>ASQHHHHHHVTNDCPVTITTTPPQTVGVSSTTPIGFSAKVTTSDQCIKAGAKVWLWGTGPANKWVLQHAKVAKQKYTLNPSIDGGADFVNQGTDAKIYKKLTSGNKFLNASVSVNPKTQVLIPGEYTM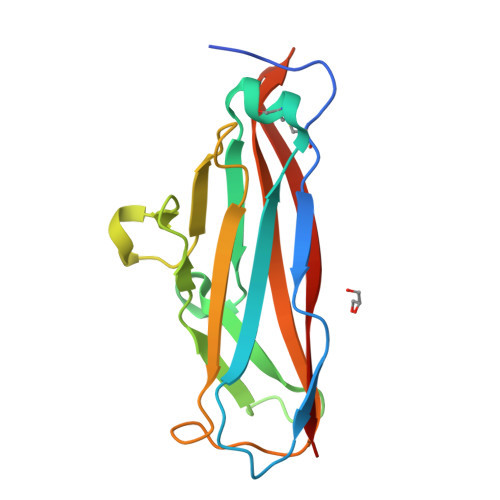ILHAAVDFDNKQGGASQQTTQTIRLTVT[2x]>[5x]GSAAAQDMVSPPPPIADEPLTVNTGIYLIESYSLDDCAETFKVNAFLSLSWKDRRLAFDPVRSGVRVKTYEPEAIWIPEIRFVNVENARDADVVDISVSPDGTVQYLERFSARVLSPLDFRRYPFDSQTLHIYLIVRSVDTRNIVLAVDLEKVGKNDDVFLTGWDIESFTAVVKPANFALEDRLESKLDYQLRISRQYFSYIPNIILPMLFILFISWTAFWSTSYEANVTLVVSTLIAHIAFNILVET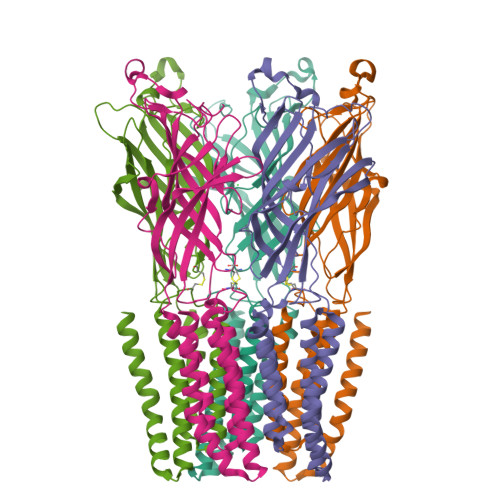NLPCTPYMTYTGAIIFMIYLFYFVAVIEVTVQHYLKVESQPARAASITRASRIAFPVVFLLANIILAFLFFGF>GPGSELPQMVQQLNSPDQQELQSALRKLSQIASGGNEQIQAVIDAGALPALVQLLSSPNEQILQEALWALSNIASGGNEQIQAVIDAGALPALVQLLSSPNEQILQEALWALSNIASGGNEQIQAVIDAGALPALVQLLSSPNEQI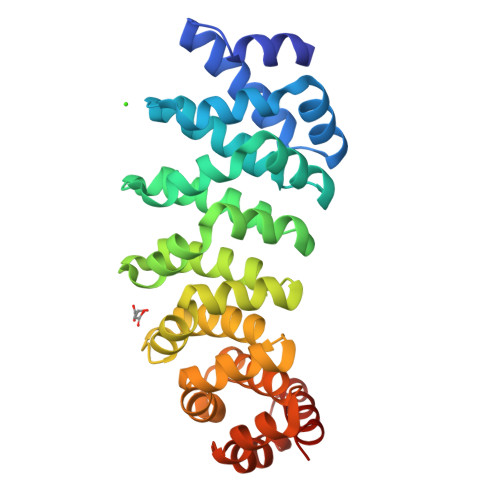LQEALWALSNIASGGNEQIQAVIDAGALPALVQLLSSPNEQILQEALWALSNIASGGNEQIQAVIDAGALPALVQLLSSPNEQILQEALWALSNIASGGNEQKQAVKEAGALEKLEQLQSHENEKIQKEAQEALEKLQSH[2x]> VSKLWVPNTDFDVAANWSQNRTPCAGGAVEFPADKMVSVLVQEGHAVSDMLLPLDGELVLASGAGFGVSDVGSHLDCGAGEPAVFRDSDRFSWHDPHLWRSGDEAPGLFFVDAERVPCRHDDVFFPPSASFRVGLGPGASPVRVRSISALGRTFTRDEDLAVFLASRAGRLRFHGPGALSVGPEDCADPSGCVCGNAEAQPWICAALLQPLGGRCPQAACHSALRPQGQCCDLCGAVVLLTHGPAFDLERYRARILDTFLGLPQYHGLQVAVSKVPRSSRLREADTEIQVVLVENGPETGGAGRLARALLADVAENGEALGV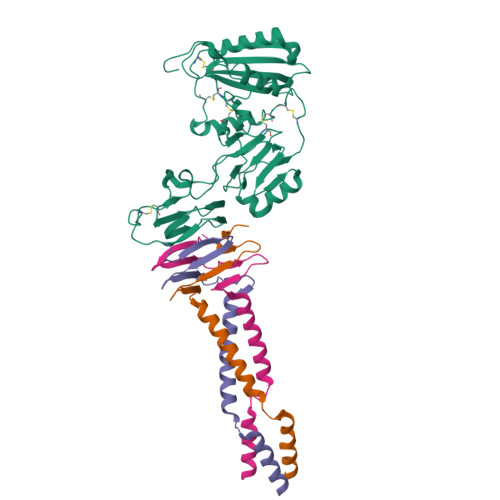LEATMRESGAHVWGSS;>GELELQRQKRSINLQQPRMATERGNLVFLTGSAQNIEFRTGSLGKIKLNDEDLSECLHQIQKNKEDIIELKGSAIGLPQNISSQIYQLNSKLVDLERKFQGLQQTVDKKV[3x]>[4x]QNSHMVKDLNLYAKELVDVVNYLMKKNQLVFSRNNKFIYVNTETIKSMLEKRNYDTVDGKLYLWRELEWIECAEDRFNKRIKIDGENMYAVVIKYSSYSILKRLYLE

In the Gram-positive pathogenic bacterium Clostridium perfringens the conjugative tetracycline resistance plasmid pCW3 is representative of a large class of closely related toxin and antibiotic resistance plasmids. In this study, we have identified TcpK, a protein encoded by a gene upstream of the oriT site and tcpM, as being a major factor required for the efficient conjugation of the pCW3 plasmid. Our data revealed that TcpK was a distantly related member of the wHTH family of DNA binding proteins. Our data suggest that its function is to decorate the origin of transfer of pCW3 and to interact specifically with sequences that are only present in this region of the plasmid.

Four identical TcpK molecules were present in the asymmetric unit, each comprising four α-helices and five β-strands. Most notably, TcpK contains a major deletion in the C-terminal region and lacks the domain responsible for the dimerization of MukF and other members of the MarR family. Macromolecular interface analysis of the crystal structure using PISA13 suggests that despite lacking the canonical MukF-like or MarR-like dimerization domain, TcpK is still predicted to form a dimer. The proposed dimer interface involves 48 residues for a total surface area of 866 Å2. These interactions are predominantly mediated through helices H1, H3 and H4. Interfacing residues in helix H1 consist of V1–N5, all of which contribute through an extensive network of hydrogen bonds and/or salt bridges. Surprisingly, the second helix of the dimer interface (helix H3), involving Y57, L58 and E61–W64, is predicted to be involved in DNA binding. Most notably, the canonical helix (H3) responsible for interacting with DNA in other wHTH superfamily members was buried at the dimer interface involving helices H1, H3 and H4’, and was hence inaccessible. In particular, the dimerization mode was incompatible with the usual arrangement of wHTH proteins in the context of binding DNA. The theoretical sedimentation coefficients for the dimer observed in the crystal structure and the corresponding monomer of TcpK were 2.2 S and 1.4 S, providing further support for a dimeric structure in solution.>[4x]GNSKSGALSKEILEELQLNTKFTEEELSSWYQSFLKECPSGRITRQEFQTIYSKFFPEADPKAYAQHVFRSFDANSDGTLDFKEYVIALHMTSAGKTNQKLEWAFSLYDVD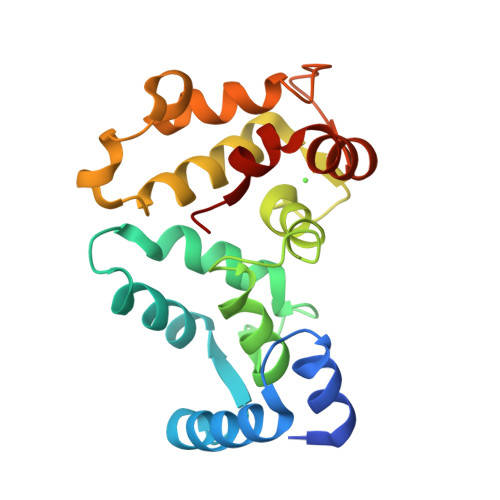GNGTISKNEVLEIVTAIFKMISPEDTKHLPEDENTPEKRAEKIWGFFGKKDDDKLTEKEFIEGTLANKEILRLIQFEP[(5-CHLORO-PYRIDIN-2-YLAMINO)-PHOSPHONO-METHYL]-PHOSPHONIC ACID | C6 H9 Cl N2 O6 P2 | 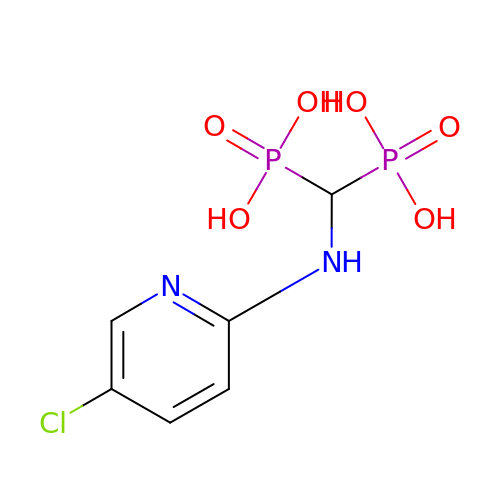BNMYZGAZFGNKTH-UHFFFAOYSA-N>MGSSHHHHHHSSGLVPRGSHQDPWKLSADKPDSNNYYGETVANGMIGIISSPEPLKVKEVVLAGTYDIYKRGRVSSFIPNYNLLNMKLAFNGESVQTYNINNYKQELDMRNGAFTGSFQFKDLATVTYSYYALRHLPHCIMMVVNINTQKDTEINVENLLETPSSLNNQQNYFQNITNTHVNIPLLTSVAFTPTGRSKIAVSNTFLFDEGKKLQPEILHRMNDADMHAMSFDKKIKAGKTYSFALIGSLISSDHINDPYNEAERLTIYAALEGKSRLLNRHMQEWNSLWQSDIQVEGDPQAQQDIRSMLYHLYSFTRKSTSLSPSPMGLSGLGYNGHVFWDTEIWMFPPMLLLHPEIAKSMIEYRYQRLDAARKKAAIYGYDGAMFPWESADSGAEETPVNALTGAFEHHVTGDVAIAAWQYYLVTGDKEWLKEKGWPILKATAEFWASRVEKNDKGEYEIKNVVAADEWAENIDNNAYTNGTAIRNLQYASKCATVLGVIAPKEWTLIADKILISKMSNGVTREHDSYTDQNIKQADANLLAYPLKLITDKEQIERDLKYYQTKIPQSDTPAMTQAIFSLLYSRLEDSDQAYHWFKDAYQPNLNPPFRVISECKGGTNPYFSTGAGGVLQAVIMGFGGLDIDAAGGIKQVKSVLPKNWKKLTITGIGIEKKTFVLTH[3x]

In this study, we use biochemical experiments and X-ray crystallography to examine the function and structure of a GH65 enzyme from Flavobacterium johnsoniae (FjGH65A) that shows low amino acid sequence homology to reported GH65 enzymes. We found that FjGH65A does not exhibit phosphorolytic activity, but it does hydrolyze kojibiose (α-1,2-glucobiose) and oligosaccharides containing a kojibiosyl moiety without requiring inorganic phosphate. In addition, stereochemical analysis demonstrated that FjGH65A catalyzes this hydrolytic reaction via an anomer-inverting mechanism. Moreover, FjGH65A had the general base catalyst Glu616 instead, which is required to activate a nucleophilic water molecule. These results indicate that FjGH65A is an α-1,2-glucosidase and is the first bacterial GH found in the GH65 family.

We determined the structure of the enzyme in unliganded form and in complex with glucose at 1.54 and 1.40 Å resolutions, respectively. The crystal structure of FjGH65A was solved using the single-wavelength anomalous dispersion method using a KAuCl4-soaked crystal because the molecular replacement method using the reported structures of GH65 GPs failed. The FjGH65A crystals belong to the space group C2 and contain three monomers (named MolA, MolB, and MolC) in the asymmetric unit. All GH65 enzymes of known structure were dimers, and the amino acid residues responsible for hexamer formation in FjGH65A were not conserved in any reported GH65 enzymes. The monomer of FjGH65A comprises four regions as follows: an N-terminal β-sandwich domain (N-domain, residues 23–258), a helical linker region (residues 259–294), an (α/α)6-barrel catalytic domain (residues 301–641), and a C-terminal β-sheet domain (C-domain, residues 295–300 and 642–681). Although the structure of the FjGH65A N-domain is similar to those of the reported GH65 GPs, a loop (residues 71–78) in the N-domain is shorter than the corresponding region (residues 62–79) in LbMP. The loop is located in the interface of the “dimer of trimers” and is suggested to be involved in the hexamer formation of the FjGH65A. All the GH65 GPs whose structure has yet been determined to possess a phosphate-binding site consisting of lysine, histidine, and two serine residues. In FjGH65A, the two serine residues are replaced by Pro575 and Ala576, and the histidine and lysine residues are replaced by Phe625 and Met330. Instead, FjGH65A has Glu616 in the sterically similar position as the phosphate-binding site in GH65 GPs.> GCACUAGAUCGGAUG;> ATCCGATGGAT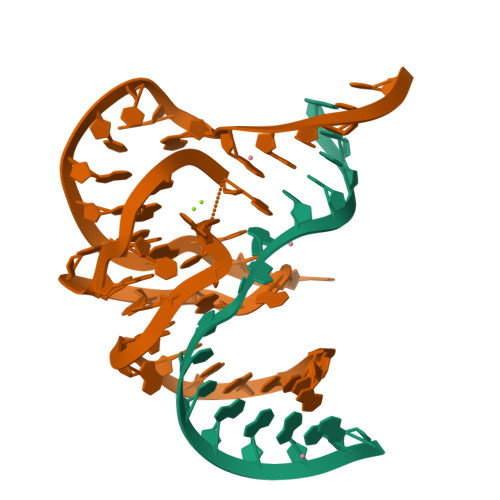CATAACGGTCGGAGGGGTTTGCCGTTTAAGTGCC> IGIGPSSSHTVGPM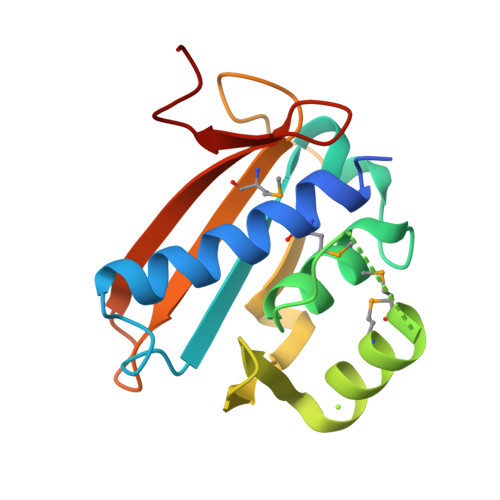LAANAFLQLLEQKNLFDKTQRVKVELYGSLALTGKGHGTDKAILNGLENKAPETVDPASMIPRMHEILDSNLLNLAGKKEIPFHEATDFLFLQKELLPKHSNGMRFSAFDGNANLLIEQVYYSIGGGFITTEEDFDK> GMINMKVAISMDVDKISNSFEDCKYFLIVRIDDNEVKSTKVIFNDESGKKSIVKENVNAIICKNISEENYKKFSKKIEIYHAEGDD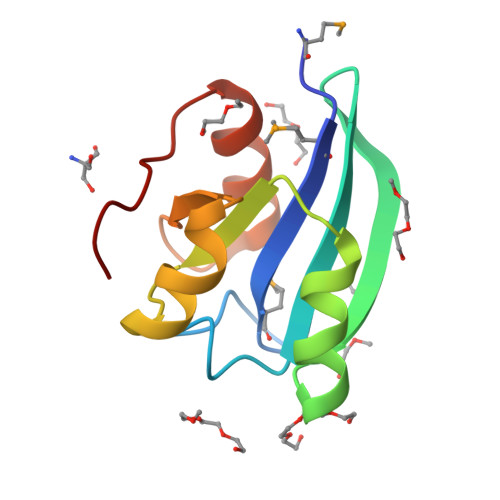VDKNISLFIEGELSKISNP>[2x]GSMPPQLHNGLDFSAKVIQGSLDSLPQEVRKFVEGNAQLCQPEYIHICDGSEEEYGRLLAHMQEEGVIRKLKKYDNCWLALTDPRDVARIESKTVIITQEQRDTVPIPKSGQSQLGRWMSEEDFEKAFNARFPGCMKGRTMYVIPFSMGPLGSPLAKIGIELTDSPYVVASMRIMTRMGTSVLEALGDGEFIKCLHSVGCPLPLKKPLVNNWACNPE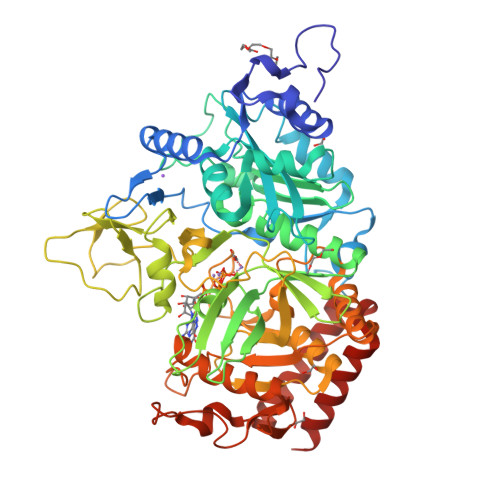LTLIAHLPDRREIISFGSGYGGNSLLGKKCFALRIASRLAKEEGWLAEHMLILGITNPEGKKKYLAAAFPSACGKTNLAMMNPTLPGWKVECVGDDIAWMKFDAQGNLRAINPENGFFGVAPGTSVKTNPNAIKTIQKNTIFTNVAETSDGGVYWEGIDEPLAPGVTITSWKNKEWRPQDEEPCAHPNSRFCTPASQCPIIDPAWESPEGVPIEGIIFGGRRPAGVPLVYEALSWQHGVFVGAAMRSEATAGAEHKGKVIMHDPFAMRPFFGYNFGKYLAHWLSMAHRPAAKLPKIFHVNWFRKDKNGKFLWPGFGENSRVLEWMFGRIEGEDSAKLTPIGYVPKEDALNLKGLGDVNVEELFGISKEFWEKEVEEIDKYLEDQVNADLPYEIERELRALKQRISQM>GSMPMYEVQWKVVEESNGNNYSYIDPTQLPYDHKWEFPRNRLSFGKTLGAGAFGKVVEATAQGLIKSDAAMTVAVKMLKPSAHSTEREALMSELKVLSYLGNHENIVNLLGACTHGGPTLVITEYCCYGDLLNFLRRKR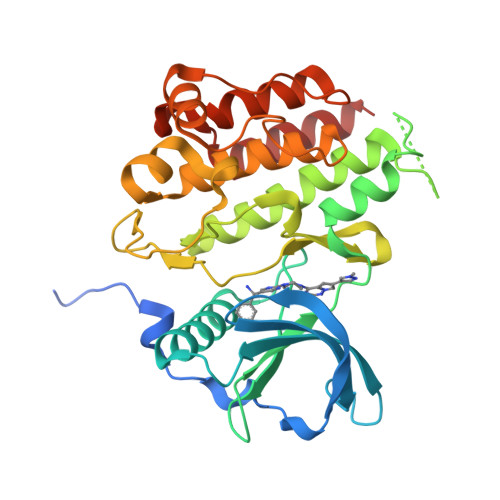DEFVPYKVAPEDLYKDFLTLEHLLSFSYQVAKGMAFLASKNCIHRDLAARNILLTHGNITKICDFGLARDIKNDSNYVDKGNARLPVKWMAPESIFNSVYTFESDVWSYGIFLWELFSLGSSPYPGMPVDSKFYKMIKEGFRMSSPEYAPAEMYDIMKTCWDADPDKRPTFKQIVQDIEKQISESTNH[2x]[3-[5-[5-(dimethylcarbamoyl)pyridin-3-yl]-1H-pyrrolo[2,3-b]pyridin-3-yl]-4-methoxy-phenyl] ethanesulfonate | C24 H24 N4 O5 S | 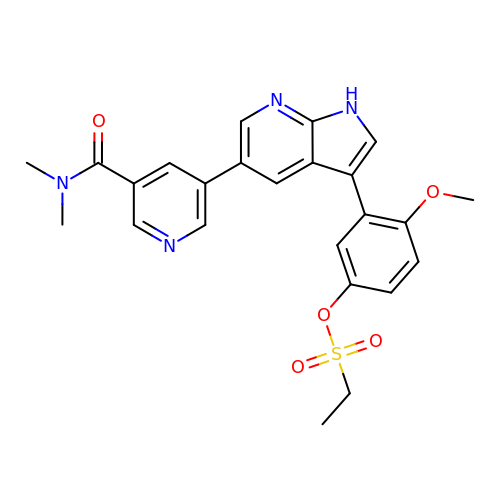BNKVNKZWIDKSEP-UHFFFAOYSA-N> MSFNANLDTLYRQVIMDHYKNPRNKGVLNDSIVVDMNNPTCGDRIRLTMKLDGDIVEDAKFEGEGCSISMASASMMTQAIKGKDIETALSMSKIFSDMMQGKEYDDSIDLGDIEALQGVSK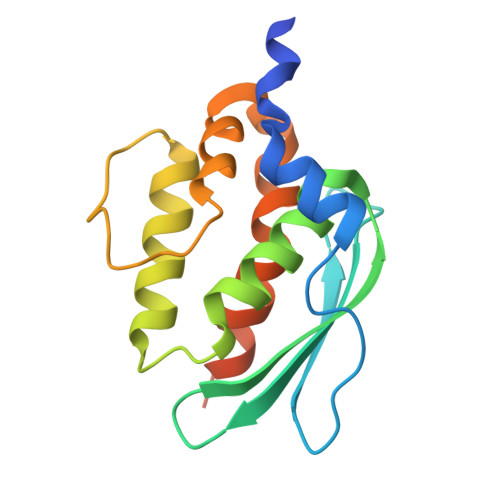FPARIKCATLSWKALEKGVAKEEGGNLEHHHHHH> GSSSGQSNNNSDTCAEFRIKYVGAIEKLKLSEGKGLEGPLDLINYIDVAQ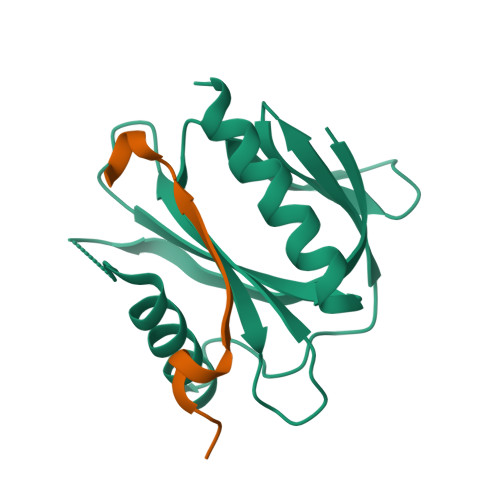QDGKLPFVPPEEEFIMGVSKYGIKVSTSDQYDVLHRHALYLIIRMVCYDDGLGAGKSLLALKTTDASNEEYSLWVYQCNSLEQAQAICKVLSTAFDSVLTSEKP;> GPLGSQSHFIPALFRPSPLERIKTNVINPAYATE> ADIFDSFELLYDRPGEPMINTKGEDKVLFELTEQFLTPEYANNGLELNNRFGDEEEVSRKIILKNLDKIPEFPKAKQLPNDADFSLFLPSHQEMANEVIDVLMSVTENQLQELLSTCVYARINLNPQLFNYCYTVAIMHRRDTGKVRVQNYAEIFPAKFLDSQVFTQAREAAAVIPKTIPRTPIIIPRDYTATDLEEEHRLAYWREDLGINLHHWHWHLVYPFSASDEKIVAKDRRGELFFYMHQQIIARYNCERLCNSLKRVKKFSDWREPIPEAYYPKLDSLTSARGWPPRQAGMRWQDLKRPVDGLNVTIDDMERYRRNIEEAIATGNVILPDKSTKKLDIDMLGNMMEASVLSPNRDLYGSIHNNMHSFSAYMHDPEHRYLESFGVIADEATTMRDPFFYRVHAWVDDIFQSFKEAPHNVRPYSRSQLENPGVQVTSVAVESAGGQQNVLNTFWMQSDVNLSKGLDFSDRGPVYARFTHLNHRPFRYVIKANNTASARRTTVRIFIAPKTDERNLPWALSDQRKMFIEMDRFVVPLSAGENTITRQSTESSLTIPFEQTFRDLSIQGSDPRRSELAAFNYCGCGWPQHMLVPKGTVGGVAYQLFVMLSNYELDKIEQPDGRELSCVEASMFCGLKDKKYPDARPMGYPFDRPSNSATNIEDFSAMSNMGLQDIVIKLSDVTEPNPRNPPA;> TDAKNNLLYFFDRPNEPCFMQKGEDKVVFEIPDHYYPDKYKSLSNTLSNRFGNEATKRIPIRNITLPNLEVPMQLPYNDQFSLFVPKHRTMAAKLIDIFMGMRDVEDLQSVCSYCQLRINPYMFNYCLSVAILHRPDTKGLSIPTFAETFPDKFMDSKVFLRAREVSNVVISGSRMPVNVPINYTANTTEPEQRVAYFREDIGINLHHWHWHLVYPFDSADRSIVNKDRRGELFYYMHQQIIGRYNVERMCNGLPQVKPFSDFSAPIEEGYFPKLDSQVASRTWPPRFAGSVFRNLDRTVDQVKIDVRKLFTWRDQFLEAIQKMAIKMPNGRELPLDEVTGIDMLGNLMESSIISPNRGYYGDLHNMGHVFAAYTHDPDHRHLEQFGVMGDSATAMRDPFFYRWHRFVDDVFNIYKEKLTPYTNERLDFPGVRVSSVGIEGARPNTLRTLWQQSTVELGRGLDFTPRGSVLARFTHLQHDEFQYVIEVNNTTGGNLMGTVRIFMAPKVDDNGQPMSFNKQRRLMIELDKFSQALRPGTNTIRRRSVDSSVTIPYERTFRNQSE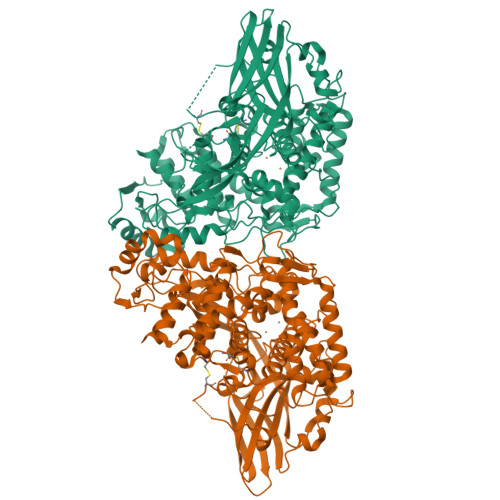RPGDPGTAGAAEFDFCGCGWPHHMLIPKGTAQGYPVVLFVMISNWNNDRIEQDLVGSCNDAASYCGIRDRKYPDKQAMGYPFDRKMANDAATLSDFLRPNMAVRDCSIQFSDTTVERGQQG>ADSAPTSQIGPTAEAYIVSHPDKVGEVVATYLAEHPEFLVAASETLHQRQQIAQQQAYVQLALQYRAELLSSSSPSVGPNEAKAAVVMFFDYQCSWC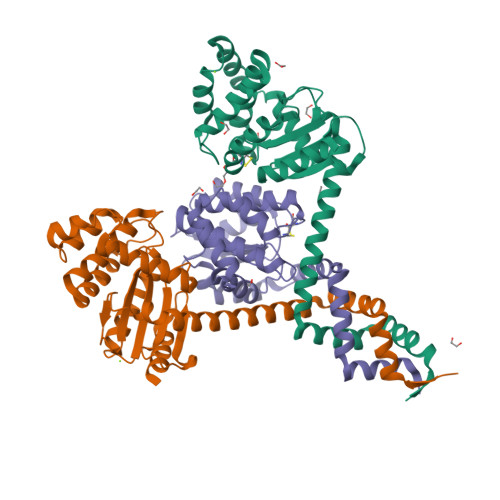SKMAPVVENLIKANPDTRFIFKEFPIFSSRWPVSGLAARVGEQVWLTQGGAKYLDWHNALYATGKVEGALTEHDVYTLAQHYLTPTQLAAVKEAQSSGAVHDALLTNQALAQHMDFSGTPAFVVMPQTQDGDVKRVTVIPGSTTQDMLQMAIQKAKG[6x]Imp-L2 can bind human IGF-1, IGF-2, insulin, and DILP5 with nM affinities, it counteracts insulin signalling in Drosophila being essential for resistance to starvation, while its overexpression leads to an extension of the lifespan. Here, we report the crystal structures of the Drosophila Imp-L2 protein in its apo-form, and in holo-complexes with insect DILP5 and human IGF-1. The three-dimensional characterisation of the Imp-L2 IBP in its free and hormone-complex forms revealed its fold and hormone-binding mode that are entirely different from, and unrelated to, IGFBP-1-6. The apo-Imp-L2 consists of two, similar, immunoglobulin-(Ig)-like fold domains, each of them with two-sandwiched layers of ~6–7 anti-parallel β-strands.

The human IGF-1:Imp-L2 complex also reveals a dimer that is very similar to DILP5:Imp-L2 quaternary arrangement (~0.89 Å rms between Cα atoms of these complexes), and the overall IGF-1 and DILP5 Imp-L2-binding modes are very similar as well. However, a higher resolution of the X-ray data allowed here an unambiguous tracing of the IGF-1 Gly1-Cys6 N-terminus that corresponds to a partially disordered N-end of the DILP5 B-helix. The IGF-1:Imp-L2 complex confirms the nature of the hormone:Imp-L2 interactions observed in the DILP5:Imp-L2 complex. The IGF-I R-like state is stabilised by a firm anchoring of the hormone Gly1 NH2-terminus onto Imp-L2 surface by 1Gly-NH2—CO Met214 hydrogen bond (3.2 Å), and close Van der Waals contacts of IGF-1 Cys6–Cys48 disulphide with the side chain of Imp-L2 Met214. Hydrogen bonds between Impl-L2 Asn216 -ND2 and -OE1 Glu9 of IGF-1 augment the conformational stability of this region. Here, the N-(1–30) and C-(Pro236-Leu238)-termini of the Imp-L2 move apart, contributing to the expansion of the id-β-sheet surface by accommodating the Asp160-Met162 peptide as a more integral part of this β-sheet. A hydrogen bond between hydroxyl of Tyr235 and peptide carbonyl of IGF-1 Cys52 is formed in this process as well. Moreover, as the CysB7-CysA7 disulphide in insulin adjusts easily to R-state α-helix, its hIGF-1 counterpart—Cys6-Cys48 cystine—isomerises in this transition, pulling Cα atom of Cys48 by ~2.7 Å, and bringing the whole Cys6–Cys48 bridge into a close contact with the Imp-L2 surface. The importance of the Imp-L2 C-terminus in insulin-like hormone binding is even more evident in the hIGF-1:Imp-L2 complex, in which the 51–53 linker of the hIGF-1 A-helices is hydrogen-bonded to the Imp-L2 by 52Cys CO-HN Leu238 (2.8 Å), and Ser51 OG-OC Pro236 (2.9 Å) interactions. Here, we show that sole protein-protein interactions, unlike the insulin organic ligand-induced ones, are sufficient to facilitate and stabilize a full (B1–B19) helix formation in IGF-1 and DILP5.

> RAVDLVDDSNDVDNSIEAEEEKPRNRAFEADWLKFTKTPPTKLQQADGATIEIVCEMMGSQVPSIQWVVGHLPRSELDDLDSNQVAEEAPSAIVRVRSSHIIDHVLSEARTYTCVGRTGSKTIYASTVVHPPRSSRLTPEKTYPGAQKPRIIYTEKTHLDLMGSNIQLPCRVHARPRAEITWLNNENKEIVQGHRHRVLANGDLLISEIKWEDMGNYKCIARNVVGKDTADTFVYPVLNEED;> GPETLCGAELVDALQFVCGDRGFYFNKPTGYGSSSRRAPQTGIVDECCFRSCDLRRLEMYCAPLKPAKSA> MATPSFGNSSPQLTFTHVANFMNDAAADVSAVDAKQLAQIRQFLKANKTNLIESLNTIRQNVTSSGDHNKLRSTIANLLQINVDNDPFFAQSEDLSHAVEFFMSERSSRLHIVYSLLVNPDIDLETYSFIDNDRFNVVGKLISIISSVIQNYDIITASSLAHDYNNDQDMFTIVSLVQLKKFSDLKFILQILQILNLMILNTKVPVDIVNQWFLQYQNQFVEFCRNINSTDKSIDTSSLQLYKFQNFQDLSYLSETLISRISSLFTITTILILGLNTSIAQFDIQSPLYMDTETFDTVNSALENDVATNIVNEDPIFHPMIHYSWSFILYYRRALQSSESFDDSDITKFALFAESHDVLQKLNTLSEILSFDPVYTTVITVFLEFSLNFIPITASTSRVFAKIISKAPEQFIENFLTNDTFEKKLSIIKAKLPLLNESLIPLINLALIDTEFANFELKDICSFAVTKSSLNDLDYDLIADTITNSSSSSDIIVPDLIELKSDLLVAPPLENENSNCLLSIPKSTKGKILTIKQQQQQQQQQNGQQPPTTSNLIIFLYKFNGWSLVGRILQNLLHSYMEKGTQLDDLQHELMISIIKLVTNVVDPKTSIEKSSEILSYLSNSLDTSASTINGASIIQVIFEIFEISLQRKDYTSIVQCCEFMTMLTPNYLHLVSSYLNKSDLLDKYGKTGLSNMILGSVELSTGDYTFTIQLLKLTKVFIRESLSLKNIHISKRSKIDIINKLILHAIHIFESYYNWKYNNFLQKFEIAFHLTLIFYDVLHDVFTINPHQKDQLIISSSANKLLQLFLTPMDSIDLAPNTLTNILISPLNTTTKILGDKILGNLYSKVMNNSFKLCTLLIAIRGSNRDLKPSNLEKLLFINSSKLVDVYTLPSYVHFKVQIIELLSYLVEAPWNDDYPFLLSFLGEAKSMAFLKEVLSDLSSPVQDWNLLRSLYIFFTTLLESKQDGLSILFLTGQFASNKKINDESSIDKKSSILTVLQKNSLLLDSTPEEVSCKLLETITYVLNTWTNSKIFIKDPKFVNSLLAKLKDSKKLFQKKENLTRDETVSLIKKYKLISRIVEIFALCIYNSTDSNSEILNFLNQEDLFELVHHFFQIDGFNKTFHDELNLKFKEKWPSLELQSFQKIPLSRINENENFGYDIPLLDIVLKADRSWNEPSKSQTNFKEEITDASLNLQYVNYEISTAKAWGALITTFVKRSTVPLNDGFVDLVEHFLKLNIDFGSDKQMFTQIYLERIELSFYILYSFKLSGKLLKEEKIIELMNKIFTIFKSGEIDFIKNIGKSLKNNFYRPLLRSVLVLLELVSSGDRFIELISDQLLEFFELVFSKGVYLILSEILCQINKCSTRGLSTDHTTQIVNLEDNTQDLLLLLSLFKKITNVNPSKNFNVILASSLNEVGTLKVILNLYSSAHLIRINDEPILGQITLTFISELCSIEPIAAKLINSGLYSVLLESPLSVAIQQGDIKPEFSPRLHNIWSNGLLSIVLLLLSQFGIKVLPETCLFVSYFGKQIKSTIYNWGDNKLAVSSSLIKETNQLVLLQKMLNLLNYQELFIQPKNSDDQQEAVELVIGLDSEHDKKRLSAALSKFLTHPKYLNSRIIPTTLEEQQQLEDESSRLEFVKGISRDIKALQDSLFKDV;>[2x]MACLSRIDANLLQYYEKPEPNNTVDLYVSNNSNNNGLKEGDKSISTPVPQPYGSEYSNCLLLSNSEYICYHFSSRSTLLTFYPLSDAYHGKTINIHLPNASMNQRYTLTIQEVEQQLLVNVILKDGSFLTLQLPLSFLFSSANTLNGEWFHLQNPYDFTVRVPHFLFYVSPQFSVVFLEDGGLLGLKKVDGVHYEPLLFNDNSYLKSLTRFFSRSSKSDYDSVISCKLFHERYLIVLTQNCHLKIWDLTSFTLIQDYDMVSQSDSDPSHFRKVEAVGEYLSLYNNTLVTLLPLENGLFQMGTLLVDSSGILTYTFQNNIPTNLSASAIWSIVDLVLTRPLELNVEASYLNLIVLWKSGTASKLQILNVNDESFKNYEWIESVNKSLVDLQSEHDLDIVTKTGDVERGFCNLKSRYGTQIFERAQQILSENKIIMAHNEDEEYLANLETILRDVKTAFNEASSITLYGDEIILVNCFQPYNHSLYKLNTTVENWFYNMHSETDGSELFKYLRTLNGFASTLSNDVLRSISKKFLDIITGELPDSMTTVEKFTDIFKNCLENQFEITNLKILFDELNSFDIPVVLNDLINNQMKPGIFWKKDFISAIKFDGFTSIISLESLHQLLSIHYRITLQVLLTFVLFDLDTEIFGQHISTLLDLHYKQFLLLNLYRQDKCLLAEVLLKDSSEFSFGVKFFNYGQLIAYIDSLNSNVYNASITENSFFMTFFRSYIIENTSHKNIRFFLENVECPFYLRHNEVQEFMFAMTLFSCGNFDQSYEIFQLHDYPEAINDKLPTFLEDLKSENYHGDSIWKDLLCTFTVPYRHSAFYYQLSLLFDRNNSQEFALKCISKSAEYSLKEIQIEELQDFKEKQHIHYLNLLIHFRMFEEVLDVLRLGHECLSDTVRTNFLQLLLQEDIYSRDFFSTLLRLCNAHSDNGELYLRTVDIKIVDSILSQNLRSGDWECFKKLYCFRMLNKSERAAAEVLYQYILMQADLDVIRKRKCYLMVINVLSSFDSAYDQWILNGSKVVTLTDLRDELRGL;>MTIDDSNRLLMDVDQFDFLDDGTAQLSNNKTDEEEQLYKRDPVSGAILVPMTVNDQPIEKNGDKMPLKFKLGPLSYQNMAFITAKDKYKLYPVRIPRL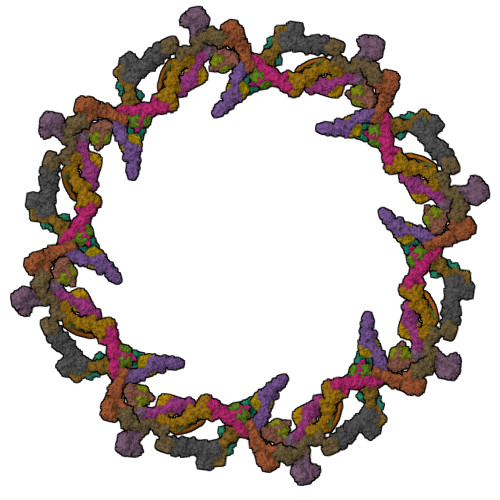DTSKEFSAYVSGLFEIYRDLGDDRVFNVPTIGVVNSNFAKEHNATVNLAMEAILNELEVFIGRVKDQDGRVNRFYELEESLTVLNCLRTMYFILDGQDVEENRSEFIESLLNWINRSDGEPDEEYIEQVFSVKDSTAGKKVFETQYFWKLLNQLVLRGLLSQAIGCIERSDLLPYLSDTCAVSFDAVSDSIELLKQYPKDSSSTFREWKNLVLKLSQAFGSSATDISGELRDYIEDFLLVIGGNQRKILQYSRTWYESFCGFLLYYIPSLELSAEYLQMSLEANVVDITNDWEQPCVDIISGKIHSILPVMESLDSCTAAFTAMICEAKGLIENIFEGEKNSDDYSNEDNEMLEDLFSYRNGMASYMLNSFAFELCSLGDKELWPVAIGLIALSATGTRSAKKMVIAELLPHYPFVTNDDIEWMLSICVEWRLPEIAKEIYTTLGNQMLSAHNIIESIANFSRAGKYELVKSYSWLLFEASCMEGQKLDDPVLNAIVSKNSPAEDDVIIPQDILDCVVTNSMRQTLAPYAVLSQFYELRDREDWGQALRLLLLLIEFPYLPKHYLVLLVAKFLYPIFLLDDKKLMDEDSVATVIEVIETKWDDADEKSSNLYETIIEADKSLPSSMATLLKNLRKKLNFKLCQAFM[2x];>[2x]SIWGLVNEEDAEIDEDDLSKQEDGGEQPLRKVRTLAQSKPSDKEVILKTDGTFGTLSGKDDSIVEEKAYEPDLSDADFEGIEASPKLDVSKDWVEQLILAGSSLRSVFATSKEFDGPCQNEIDLLFSECNDEIDNAKLIMKERRFTASYTFAKFSTGSMLLTKDIVGKSGVSIKRLPTELQRKFLFDDVYLDKEIEKVTIEARKSNPYPQISESSLLFKDALDYMEKTSSDYNLWKLSSILFDPVSYPYKTDNDQVKMALLKKERHCRLTSWIVSQIGPEIEEKIRNSSNEIEQIFLYLLLNDVVRASKLAIESKNGHLSVLISYLGSNDPRIRDLAELQLQKWSTGGCSIDKNISKIYKLLSGSPFEGLFSLKELESEFSWLCLLNLTLCYGQIDEYSLESLVQSHLDKFSLPYDDPIGVIFQLYAANENTEKLYKEVRQRTNALDVQFCWYLIQTLRFNGTRVFSKETSDEATFAFAAQLEFAQLHGHSLFVSCFLNDDKAAEDTIKRLVMREITLLRASTNDHILNRLKIPSQLIFNAQALKDRYEGNYLSEVQNLLLGSSYDLAEMAIVTSLGPRLLLSNNPVQNNELKTLREILNEFPDSERDKWSVSINVFEVYLKLVLDNVETQETIDSLISGMKIFYDQYKHCREVAACCNVMSQEIVSKILEKNNPSIGDSKAKLLELPLGQPEKAYLRGEFAQDLMKCTYKI;>MVVIANAHNELIHDAVLDYYGKRLATCSSDKTIKIFEVEGETHKLIDTLTGHEGPVWRVDWAHPKFGTILASCSYDGKVLIWKEENGRWSQIAVHAVHSASVNSVQWAPHEYGPLLLVASSDGKVSVVEFKENGTTSPIIIDAHAIGVNSASWAPATIEEDGEHNGTKESRKFVTGGADNLVKIWKYNSDAQTYVLESTLEGHSDWVRDVAWSPTVLLRSYLASVSQDRTCIIWTQDNEQGPWKKTLLKEEKFPDVLWRASWSLSGNVLALSGGDNKVTLWKENLEGKWEPAGEVHQ[2x];>[2x]MQPFDSGHDDLVHDVVYDFYGRHVATCSSDQHIKVFKLDKDTSNWELSDSWRAHDSSIVAIDWASPEYGRIIASASYDKTVKLWEEDPDQEECSGRRWNKLCTLNDSKGSLYSVKFAPAHLGLKLACLGNDGILRLYDALEPSDLRSWTLTSEMKVLSIPPANHLQSDFCLSWCPSRFSPEKLAVSALEQAIIYQRGKDGKLHVAAKLPGHKSLIRSISWAPSIGRWYQLIATGCKDGRIRIFKITEKLSPLASEESLTNSNMFDNSADVDMDAQGRSDSNTEEKAELQSNLQVELLSEHDDHNGEVWSVSWNLTGTILSSAGDDGKVRLWKATYSNEFKCMSVITAQQ;>MELSPTYQTERFTKFSDTLKEFKIEQNNEQNPIDPFNIIREFRSAAGQLALDLANSGDESNVISSKDWELEARFWHLVELLLVFRNADLDLDEMELHPYNSRGLFEKKLMQDNKQLYQIWIVMVWLKENTYVMERPKNVPTSKWLNSITSGGLKSCDLDFPLRENTNVLDVKDKEEDHIFFKYIYELILAGAIDEALEEAKLSDNISICMILCGIQEYLNPVIDTQIANEFNTQQGIKKHSLWRRTVYSLSQQAGLDPYERAIYSYLSGAIPNQEVLQYSDWESDLHIHLNQILQTEIENYLLENNQVGTDELILPLPSHALTVQEVLNRVASRHPSESEHPIRVLMASVILDSLPSVIHSSVEMLLDVVKGTEASNDIIDKPYLLRIVTHLAICLDIINPGSVEEVDKSKLITTYISLLKLQGLYENIPIYATFLNESDCLEACSFILSSLEDPQVRKKQIETINFLRLPASNILRRTTQRVFDETEQEYSPSNEISISFDVNNIDMHLIYGVEWLIEGKLYVDAVHSIIALSRRFLLNGRVKALEQFMERNNIGEICKNYELEKIADNISKDENEDQFLEEITQYEHLIKGIREYEEWQKSVSLLSSESNIPTLIEKLQGFSKDTFELIKTFLVDLTSSNFADSADYEILYEIRALYTPFLLMELHKKLVEAAKLLKIPKFISEALAFTSLVANENDKIYLLFQSSGKLKEYLDLVARTATLSN[2x];>MSEKKVHLRLRKELSVPIAVVENESLAQLSYEEESQASLMDISMEQQQLRLHSHFDNSKVFTENNRYIVKTLQTDYSSGFSNDDELNGYIDMQIGYGLVNDHKKVYIWNIHSTQKDTPYITVPFRSDDNDEIAVAPRCILTFPATMDESPLALNPNDQDETGGLIIIKGSKAIYYEDINSINNLNFKLSEKFSHELELPINSSGGEKCDLMLNCEPAGIVLSTNMGRIFFITIRNSMGKPQLKLGKLLNKPFKLGIWSKIFNTNSSVVSLRNGPILGKGTRLVYITTNKGIFQTWQLSATNSHPTKLIDVNIYEAILESLQDLYPFAHGTLKIWDSHPLQDESSQLFLSSIYDSSCNETYYILSTIIFDSSSNSFTIFSTYRLNTFMESITDTKFKPKIFIPQMENANDTNEVTSILVMFPNAVVITQVNSKLDSSYSMRRKWEDIVSLRNDIDIIGSGYDSKSLYVLTKQMGVLQFFVKENEETNSKPEVGFVKSHVDQAVYFSKINANPIDFNLPPEISLDQESIEHDLKLTSEEIFHSNGKYIPPMLNTLGQHLSVRKEFFQNFLTFVAKNFNYKISPELKLDLIEKFEILNCCIKFNSIIRQSDVLNDIWEKTLSNYNLTQNEHLTTKTVVINSPDVFPVIFKQFLNHVVFVLFPSQNQNFKLNVTNLINLCFYDGILEEGEKTIRYELLELDPMEVDTSKLPWFINFDYLNCINQCFFDFTFACEEEGSLDSYKEGLLKIVKILYYQFNQFKIWINTQPVKSVNANDNFININNLYDDNHLDWNHVLCKVNLKEQCIQIAEFYKDLSGLVQTLQTLDQNDSTTVSLYETFFNEFPKEFSFTLFEYLIKHKKLNDLIFRFPQQHDVLIQFFQESAPKYGHVAWIQQILDGSYADAMNTLKNITVDDSKKGESLSECELHLNVAKLSSLLVEKDNLDINTLRKIQYNLDTIDAEKNISNKLKKGEVQICKRFKNGSIREVFNILVEELKSTTVVNLSDLVELYSMLDDEESLFIPLRLLSVDGNLLNFEVKKFLNALVWRRIVLLNASNEGDKLLQHIVKRVFDEELPKNNDFPLPSVDLLCDKSLLTPEYISETYGRFPIDQNAIREEIYEEISQVETLNSDNSLEIKLHSTIGSVAKEKNYTINYETNTVEY[2x]>[2x]GSETYD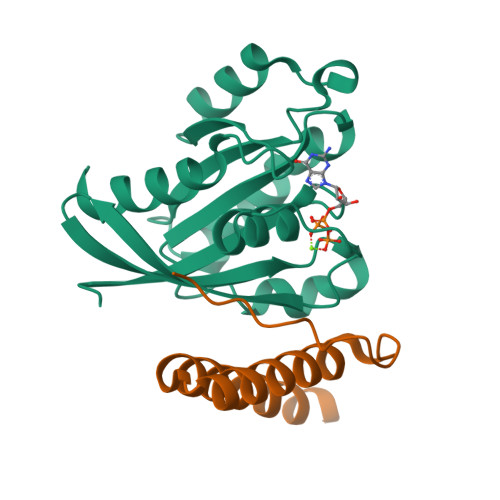FLFKFLVIGNAGTGKSCLLHQFIEKKFKDDSNHTIGVEFGSKIINVGGKYVKLQIWDTAGLERFRSVTRSYYRGAAGALLVYDITSRETYNALTNWLTDARMLASQNIVIILCGNKKDLDADREVTFLEASRFAQENELMFLETSALTGEDVEEAFVQCARKILNK;>[2x]GPLGSAEGWLPLSGGQGQSEDSDPLLQQIHNITSFIRQAKAAGRMDEVRTLQENLRQLQDEYDQQQTEK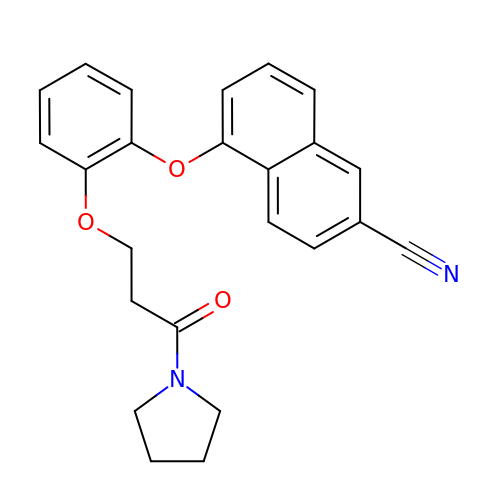5-{2-[3-oxo-3-(pyrrolidin-1-yl)propoxy]phenoxy}naphthalene-2-carbonitrile | C24 H22 N2 O3 | UTKNCYCOFRHJAD-UHFFFAOYSA-N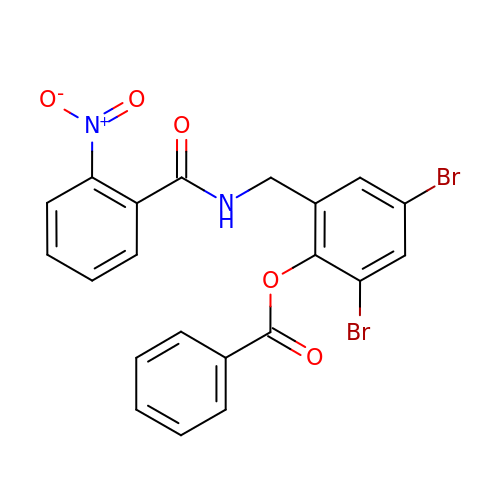2,4-dibromo-6-{[(2-nitrobenzene-1-carbonyl)amino]methyl}phenyl benzoate | C21 H14 Br2 N2 O5 | TYMXZAAQZPJROA-UHFFFAOYSA-N>[2x]PGSMTLSSNQYQLPLNVRPYTTTWCSQSPSCSNLLAIGHDTGITIYCASEEQTPGSTGLTLQELFTIQTGLPTLHLSFSSSCSYSENLHDGDGNVNSSPVYSLFLACVCQDNTVRLIITKNETIITQHVLGGKSGHHNFVNDIDIADVYSADNRLAEQVIASVGDDCTLIIWRLTDEGPILAGYPLSSPGISVQFRPSNPNQLIVGERNGNIRIFDWTLNLSAEENSQTELVKNPWLLTLNTLPLVNTCHSSGIASSLANVRWIGSDGSGILAMCKSGAWLRWNLFANNDYNEISDSTMKLGPKNLLPNVQGISLFPSLLGACPHPRYMDYFATAHSQHGLIQLINTYEKDSNSIPIQLGMPIVDFCWHQDGSHLAIATEGSVLLTRLMGFTRL;>PGSMNELKHAVVPIDLQSFCLEGTLALWVPALENDSEDDSEAIETADDNEKLFKKECVAYDAGVYTSNKSKGSQTLRWSIFQNRTLTIFDVSLNSKKEPLSKFNVKIHFPSNVMKDGVAFSFSEHSDTTIIYAITHARVLYYIRLSKTWFQLPDARLDDDWCLCYRPISFLNQKPDLMAAISTSEICVSFFNGGLTKIILNPKDASHYEQHIDDSSYLFSLKKYLSLQAFKADYRSPNTIISMIFLSTYNVLVMLSLDYKLKVLDLSTNQCVETIELSQTILPLQSFPYLTSDHTTNSFIALYYPDNSHGSFSIYKLNANAHSFKLNVVIEKGIIPPSLPDDEFIPWMLSDFQLISSEGSQSKFLLIIAWKSNLNTVIQKCNLSLDQDESFSCVWSHSLDSFSLIEKTFFDVPTNMSSGDISEIWLQHIFAHNTSIESIQVALLSFQNSSSQVSKNKLDKFGALTISELKNAVLSSIVSTIQIEPNSDLTGYDYYEYKRLLYNEWERFAKLVAYLDHF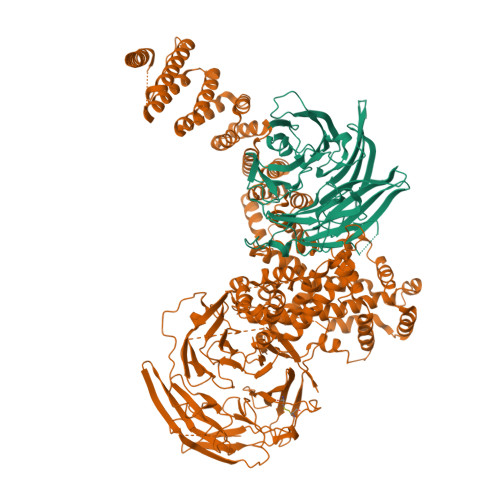GDEILSINFDPSNAVTYINYANKVAFIRDPYLIESFDEEPLTKLISSLETDDPSLIEGYQILDLGRSLHSCMSFSTLSEIRYSLRELVQDLPSYSLFDTLWVFYDKHIYPNVDPDYISTLIDTLVSLENPMRDIDSLIQRLRSFDIYNHSAQSPSLFLCASVARVLDSILKKFQVSIEGFIFLLSLITSQQDYELQSKFAGCDKLFLSLLEDWRLVSFLLENSALLLEKFEEEDVDSTNCNLNTMEALASVNTALQFFSALNYSECFSESQISPLHATVISSLSAIFIRDDTENDLVTELVEKLFLFKQYNACMQLIGWLNSDPIAVYLKALIYLKSKEAVKAVRCFKTTSLVLYSHTSQFAVLREFQEIAEKYHHQNLLSCYYLHLSKKLFEESAYIDALEFSLLADASKETDDEDLSIAITHETLKTACAAGKFDAAHVALMVLSTTPLKKSCLLDFVNQLTKQGKINQLLNYSMPTLRQDVDNLLERKAFQMINVESQPCWYNILFSWRYKHQNYRDAAAIIYEKLSRYISTTELIGKKERTFIIEHYLIVLNTLELLPKEDTWILVTDMSVDKEPDPNFLPQKLLTLDAIVAEYHLQLKDVAVQVTAEMSSAMNIDL[2x];> PGSMDQTYSLESFLNHVQKRDPNQTEFAQAVREVMTTLWPFLEQNPKYRQMSLLERLVEPERVIQFRVVWVDDRNQVQVNRAWRVQFSSAIGPYKGGMRFHPSVNLSILKFLGFEQTFKNALTTLPMGGGKGGSDFDPKGKSEGEVMRFCQALMTELYRHLGADTDVPAGDIGVGGREVGFMAGMMKKLSNNTACVFTGKGLSFGGSLIRPEATGYGLVYFTEAMLKRHGMGFEGMRVSVSGSGNVAQYAIEKAMEFGARVITASDSSGTVVDESGFTKEKLARLIEIKSSRDGRVADYAKEFGLVYLEGQQPWSVPVDIALPCATQNELDVDAAHQLIANGVKAVAEGANMPTTIEATELFQQAGVLFAPGKAANAGGVATSGLEMAQNAARLGWKAEKVDARLHHIMLDIHHACVEHGGEGEQTNYVQGANIAGFVKVADAMLAQGVI>MAMAQELTAMSAWVNQDGSTLYINSINAQGELTGSYINRAAGAACQNSPYPVNGWVFGTAISFSTKWLNSVESCNSITSWSGFYI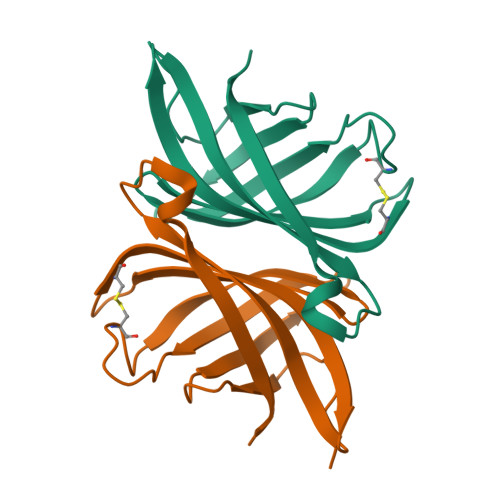NTGGQGKISTLWQLVVNGSSSPSQILKGQDVFSQTSA[4x]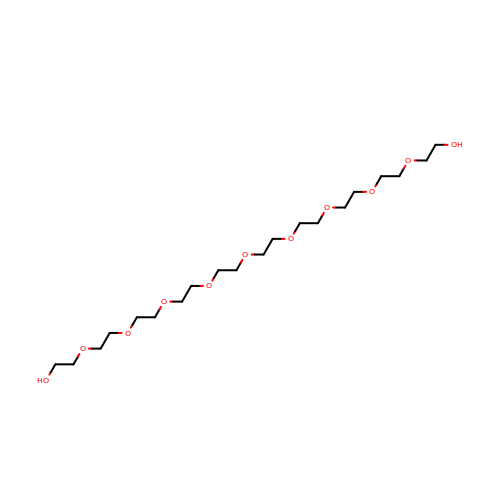3,6,9,12,15,18,21,24,27-NONAOXANONACOSANE-1,29-DIOL | C20 H42 O11 | DTPCFIHYWYONMD-UHFFFAOYSA-N> PPVVDTVHGKVLGKFVSLEGFAQPVAVFLGVPFAKPPLGSLRFAPPQPAESWSHVKNTTSYPPMCSQDAVSGHMLSELFTNRKENIPLKFSEDCLYLNIYTPADLTKRGRLPVMVWIHGGGLMVGGASTYDGLALSAHENVVVVTIQYRLGIWGFFSTGDEHSRGNWGHLDQVAALRWVQDNIANFGGDPGSVTIFGESAGGQSVSILLLSPLTKNLFHRAISESGVALLSSLFRKNTKSLAEKIAIEAGCKTTTSAVMVHCLRQKTEEELMEVTLKMKFMALDLVGDPKENTAFLTTVIDGVLLPKAPAEILAEKKYNMLPYMVGINQQEFGWIIPMQMLGYPLSEGKLDQKTATELLWKSYPIVNVSKELTPVATEKYLGGTDDPVK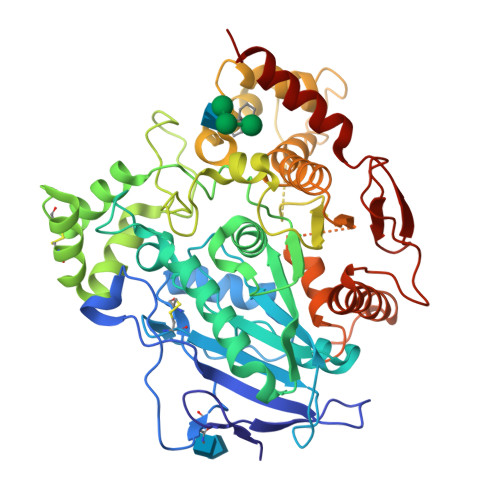KKDLFLDMLADLLFGVPSVNVARHHRDAGAPTYMYEYRYRPSFSSDMRPKTVIGDHGDEIFSVLGAPFLKEGATEEEIKLSKMVMKYWANFARNGNPNGEGLPQWPAYDYKEGYLQIGATTQAAQKLKDKEVAFWTELWAKEAAR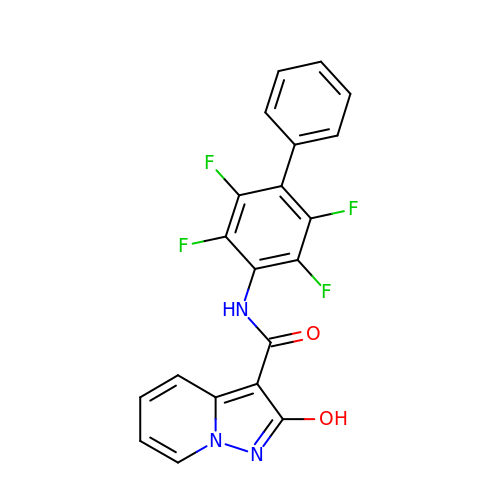2-oxidanyl-~{N}-[2,3,5,6-tetrakis(fluoranyl)-4-phenyl-phenyl]pyrazolo[1,5-a]pyridine-3-carboxamide | C20 H11 F4 N3 O2 | JIIXZPWFDKPNKW-UHFFFAOYSA-N> SFNKQWYLLANQIIQSLSKYEGGHIFEKLVDAKKQNCPDYYDVIKNPMSFSCVKTKLKKGQYGLPTEFIKDVQLIFDNCSLYNTSGSLVAITGKNIEAYF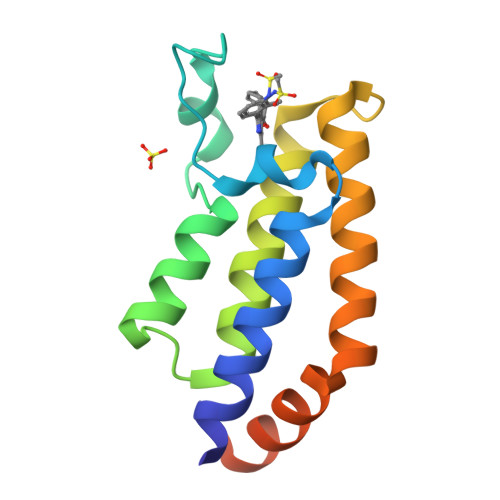NNQLIVTGYNNFVTKANTINERLQKVEDENLE> SANNPWTGFQIFLSPYYANEVAAAAKQITDPTLSSKAASVANIPTFTWLDSVAKIPDLGTYLASASALGKSTGTKQLVQIVIYDLPDRDCAAKASNGEFSIANNGQANYENYIDQIVAQIQQFPDVRVVAVIEPDSLANLVTNLNVQKCANAKTTYLASVNYALTNLAKVGVYMYMDAGHAGWLGWPANLSPAAQLFTQVWQNAGKSPFIKGLATNVANYNALQAASPDPITQGNPNYDEIHYINALAPLLQQAGWDATFIVDQGRSGVQNIRQ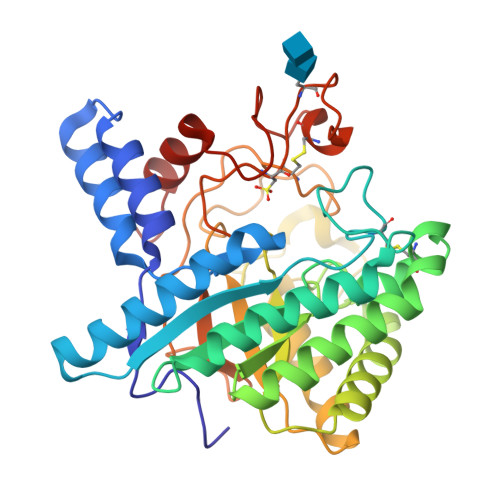QWGDWCNIKGAGFGTRPTTNTGSQFIDSIVWVKPGGESCGTSNSSSPRYDSTCSLPDAAQPAPEAGTWFQAYFQTLVSAANPPL>[3x]HMTDGERQNATEIRASVGKMIDGIGRFYIQMCTELKLSDYEGRLIQNSLTIERMVLSAFDERRNKYLEEHPSAGKDPKKTGGPIYRRVDGKWRRELILYDKEEIRRIWRQANNGDDATAGLTHMMIWHSNLNDATYQRTRALVRTGMDPRMCSLMQGSTLPRRSGAAGAAVKGVGTMVMELIRMIKRGINDRNFWRGENGRRTRIAYERMCNILKGKFQTAAQRTMVDQVRESRNPGNAEF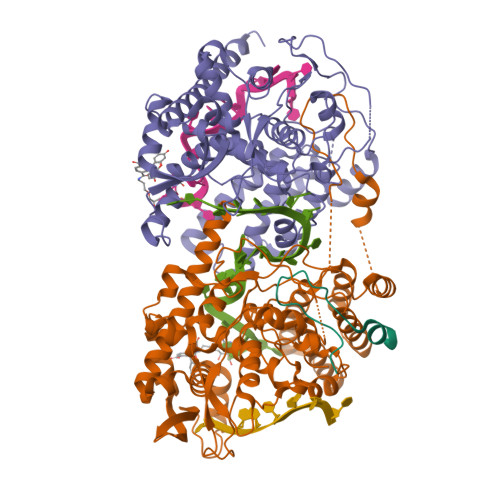EDLIFLARSALILRGSVAHKSCLPACVYGSAVASGYDFEREGYSLVGIDPFRLLQNSQVYSLIRPNENPAHKSQLVWMACHSAAFEDLRVSSFIRGTKVVPRGKLSTRGVQIASNENMETMESSTLELRSRYWAIRTRSGGNTNQQRASSGQISIQPTFSVQRNLPFDRPTIMAAFTGNTEGRTSDMRTEIIRLMESARPEDVSFQGRGVFELSDEKATSPIVPSFDMSNEGSYFFGDNAEEYDNLEHHHHHH3,4-dihydroxybenzenesulfonic acid | C6 H6 O5 S | 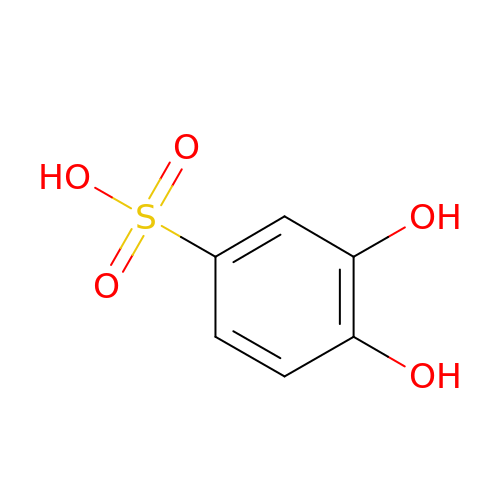LTPDITOEDOAWRU-UHFFFAOYSA-N>ATTCTFSGSNGASSASKSKTSCSTIVLSNVAVPSGTTLDLTKLNDGTHVIFSGETTFGYKEWSGPLISVSGSDLTITGASGHSINGDGSRWWDGEGGNGGKTKPKFFAAHSLTNSVISGLKIVNSPVQVFSVAGSDYLTLKDITIDNSDGDDNGGHNTDAFDIGTSTYVTISGATVYNQDDCVAVNSGENIYFSG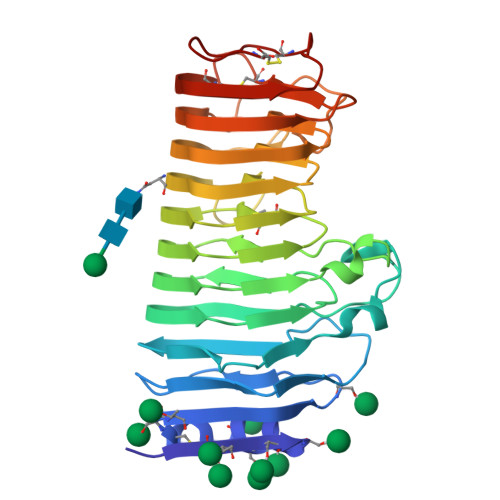GYCSGGHGLSIGSVGGRSDNTVKNVTFVDSTIINSDNGVRIKTNIDTTGSVSDVTYKDITLTSIAKYGIVVQQNYGDTSSTPTTGVPITDFVLDNVHGSVVSSGTNILISCGSGSCSDWTWTDVSVSGGKTSSKCTNVPSGASC[2x]> MNTSFGSVVPSTNFNFFKGHGNNDNTSANSTVNNSNFFLNSNETKPSKNVFMVHSTSQKKSQQPLQNLSHSPSYTENKPDKKKKYMINDAKTIQLVGPLISSPDNLGFQKRSHKARELPRFLINQEPQLEKRAFVQDPWDKANQEKMISLEESIDDLNELYETLKKMRNTERSIMEEKGLVDKADSAKDLYDAIVFQGTCLDMCPTFERSRRNVEYTVYSYEKNQPNDKKASRTKALKVFARPAAAAAPPLPSDVRPPHILVKTLDYIVDNLLTTLPESEGFLWDRMRSIRQDFTYQNYSGPEAVDCNERIVRIHLLILHIMVKSNVEFSLQQELEQLHKSLITLSEIYDDVRSSGGTCPNEAEFRAYALLSKIRDP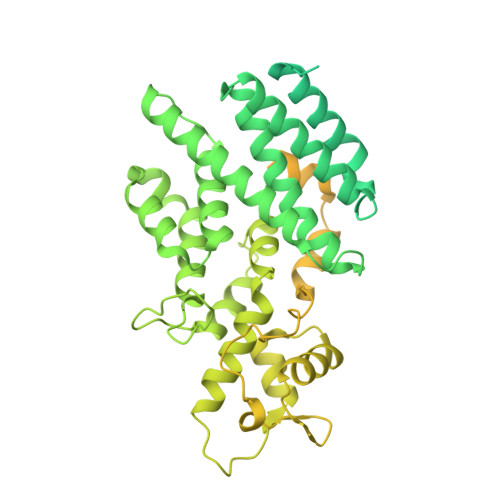QYDENIQRLPKHIFQDKLVQMALCFRRVISNSAYTERGFVKTENCLNFYARFFQLMQSPSLPLLMGFFLQMHLTDIRFYALRALSHTLNKKHKPIPFIYLENMLLFNNRQEIIEFCNYYSIEIINGDAADLKTLQHYSHKLSETQPLKKTYLTCLERRLQKTTYKGLINGGEDNLASSVYVKDPKKDRIPSIADQSFLMENFQNNYNEKLNQNSSVKPQINTSPKRVATRPNHFPFSQESKQLPQISQSHTLSTNPLLTPQVHGDLSEQKQQQIKTVTDGGSPFVFDQSAQNSTVEASKAHMISTTSNGAYDEKLSSEQEEMRKKEEQRIEEEKTQLKKKQENADKQVITEQIANDLVKEVVNSSVISIVKREFSEANYRKDFIDTMTRELYDAFLHERLYLIYMDSRAELKRNSTLKKKFFEKWQAS> PDAVFGDRVRRFQEFLDTFTSYRDSVRSIQVYNSNNAANYNDDQDDADERDLLGDDDGDDLEKEKKAASSTSLNILPHRIIISLDDLREFDRSFWSGILVEPAYFIPPAEKALTDLADSMDDVPHPNASAVSSRHPWKLSFKGSFGAHALSPRTLTAQHLNKLVSVEGIVTKTSLVRPKLIRSVHYAAKTGRFHYRDYTDATTTLTTRIPTPAIYPTEDTEGNKLTTEYGYSTFIDHQRITVQEMPEMAPAGQLPRSIDVILDDDLVDKTKPGDRVNVVGVFKSLGAGGMNQSNSNTLIGFKTLILGNTVYPLHARSTGVAARQMLTDFDIRNINKLSKKKDIFDILSQSLAPSIYGHDHIKKAILLMLMGGVEKNLENGSHLRGDINILMVGDPSTAKSQLLRFVLNTASLAIATTGRGSSGVGLTAAVTTDRETGERRLEAGAMVLADRGVVCIDEFDKMTDVDRV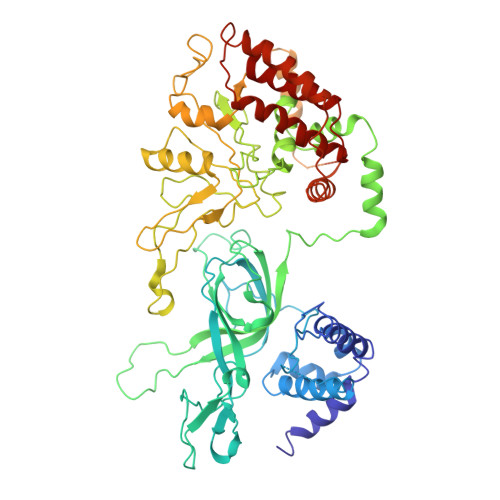AIHEVMEQQTVTIAKAGIHTTLNARCSVIAAANPVFGQYDVNRDPHQNIALPDSLLSRFDLLFVVTDDINEIRDRSISEHVLRTHRYLPPGYLEGEPVRERLNLSLAVGEDADINPEEHSNSGAGVENEGEDDEDHVFEKFNPLLQAGAKLAKNKGNYNGTEIPKLVTIPFLRKYVQYAKERVIPQLTQEAINVIVKNYTDLRNDDNTKKSPITARTLETLIRLATAHAKVRLSKTVNKVDAKVAANLLRFALL> MKIEEGKGHHHHHHMTKHSIPLHAFRNSGADARKWKGRIALLAKRGKETMRTLQFPLEMSEPEAAAINTTPFAVAYNAIEGTGKGTLFDYWAKLHLAGFRFFPSGGAATIFRQQAVFEDASWNAAFCQQSGKDWPWLVPSKLYERFTKAPREVAKKDGSKKSIEFTQENVANESHVSLVGASITDKTPEDQKEFFLKMAGALAEKFDSWKSANEDRIVAMKVIDEFLKSEGLHLPSLENIAVKCSVETKPDNATVAWHDAPMSGVQNLAIGVFATCASRIDNIYDLNGGKLSKLIQESATTPNVTALSWLFGKGLEYFRTTDIDTIMQDFNIPASAKESIKPLVESAQAIPTMTVLGKKNYAPFRPNFGGKIDSWIANYASRLMLLNDILEQIEPGFELPQALLDNETLMSGIDMTGDELKELIEAVYAWVDAAKQGLATLLGRGGNVDDAVQTFEQFSAMMDTLNGTLNTISARYVRAVEMAGKDEARLEKLIECKFDIPKWCKSVPKLVGISGGLPKVEEEIKVMNAAFKDVRARMFVRFEEIAAYVASKGAGMDVYDALEKRELEQIKKLKSAVPERAHIQAYRAVLHRIGRAVQNCSEKTKQLFSSKVIEMGVFKNPSHLNNFIFNQKGAIYRSPFDRSRHAPYQLHADKLLKNDWLELLAEISATLMASESTEQMEDALRLERTRLQLQLSGLPDWEYPASLAKPDIEVE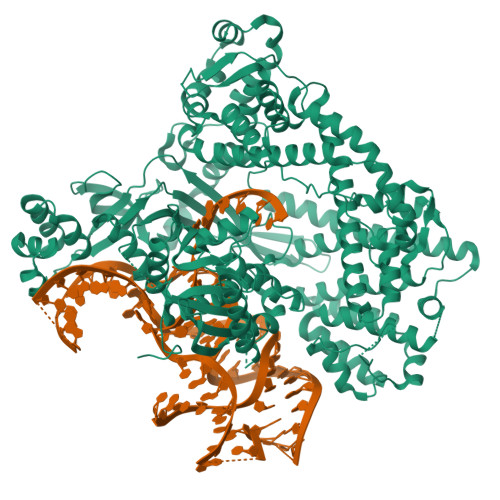IQTALKMQLAKDTVTSDVLQRAFNLYSSVLSGLTFKLLRRSFSLKMRFSVADTTQLIYVPKVCDWAIPKQYLQAEGEIGIAARVVTESSPAKMVTEVEMKEPKALGHFMQQAPHDWYFDASLGGTQVAGRIVEKGKEVGKERKLVGYRMRGNSAYKTVLDKSLVGNTELSQCSMIIEIPYTQTVDADFRAQVQAGLPKVSINLPVKETITASNKDEQMLFDRFVAIDLGERGLGYAVFDAKTLELQESGHRPIKAITNLLNRTHHYEQRPNQRQKFQAKFNVNLSELRENTVGDVCHQINRICAYYNAFPVLEYMVPDRLDKQLKSVYESVTNRYIWSSTDAHKSARVQFWLGGETWEHPYLKSAKDKKPLVLSPGRGASGKGTSQTCSCCGRNPFDLIKDMKPRAKIAVVDGKAKLENSELKLFERNLESKDDMLARRHRNERAGMEQPLTPGNYTVDEIKALLRANLRRAPKNRRTKDTTVSEYHCVFSDCGKTMHADENAAVNIGGKFIADIEK>[2x]NRAAQGDITAPGGARRLTGDQTAALRDSLSDKPAKNIIL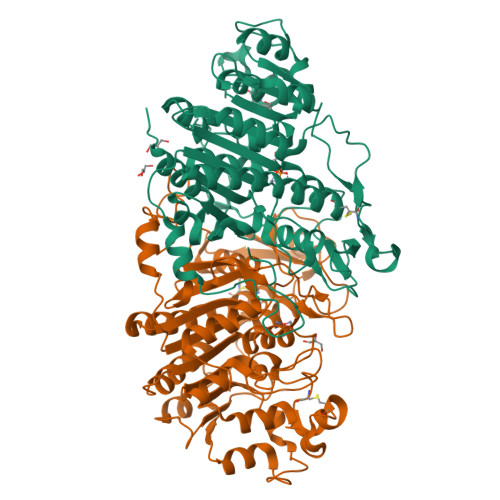LIGDGMGDSEITAARNYAEGAGGFFKGIDALPLTGQYTHYALNKKTGKPDYVTASAASATAWSTGVKTYNGALGVDIHEKDHPTILEMAKAAGLATGNVSTAELQAATPAALVAHVTSRKCYGPSATSEKCPGNALEKGGKGSITEQLLNARADVTLGGGAKTFAETATAGEWQGKTLREQAQARGYQLVSDAASLNSVTEANQQKPLLGLFADGNMPVRWLGPKATYHGNIDKPAVTCTPNPQRNDSVPTLAQMTDKAIELLSKNEKGFFLQVEGASIDKQDHAANPCGQIGETVDLDEAVQRALEFAKKEGNTLVIVTADHAHASQIVAPDTKAPGLTQALNTKDGAVMVMSYGNSEEDSQEHTGSQLRIAAYGPHAANVVGLTDQTDLFYTMKAALGLKSA> SNAPRRSIHLSNIVEQRVFEDDEIISTPKRGRSKKTVQDNDEDYSPKKSVQKTPTRTRRSSTTTKTATTPSKGITTATATPMTPSQKMKKIRAGELSPSMQQRTDLPAKDSSKSELQLAREQLHVSVVPKSLPCREREFENIYAFLEGKIQDQCGGCMYVSGVPGTGKTATVTGVIRTLQRMAKQNELPAFEYLEINGMRLTEPRQAYVQIYKQLTGKTVSWEQAHALLEKRFTTPAPRRVTTVLLVDELDILCNRRQDVVYNLLDWPTKSAAKLVVVTIANTMDLPERLLMGKVTSRLGLTRLTFQPYSHKQLQEIVTARLGGSETFKGEAVQLVARKVAAVSGDARRALDICRRATEIADTAAVKCVTMLHVQQALAEMIASAKVQAIRNCSRMEQIFLQAIAAEVTRTGVEETTFMGVYQQVETIAAFMGVTFPPPGRALRLCSKLGAERLIISEHSRNDLFQKILLNVSADDIHYALRVEEMVN;> MSASNKGGYKTPRKENLMSIENLTNSEEESEDLNTAMVGNAVESQPKVTSRRSTRRPSPTKKYQAYQKESNGKGQEERIVVNYVEMSDERSSDAEDQEEEESIEESENAARPAAKDLHLIQSEYNVAGTSMFGFNTPKKRDAMALAALNATPCTPKTPKTPRLGVKTPDTKRKKSMDQPKTPAHVRTRVKKQIAKIVADSDEDFSGDESDFRPSDEESSSSSSSSDAGNSSDNDAADDEPKTPSRARRAIVVPVLPKTPSAARLRQSARAKKSNEFVPESDGYFHSHASSKILTSDHTLDRLKNPRLAADRVFSLLSEIKTSAEHEGSINAIMEEYRSYFPKWMCILNEGFNILLYGLGSKHQLLQSFHREVLHKQTVLVVNGFFPSLTIKDMLDSITSDILDAGISPANPHEAVDMIEEEFALIPETHLFLIVHNLDGAMLRNVKAQAILSRLARIPNIHLLASIDHINTPLLWDQGKLCSFNFSWWDCTTMLPYTNETAFENSLLVQNSGELALSSMRSVFSSLTTNSRGIYMLIVKYQLKNKGNATYQGMPFRDLYSSCREAFLVSSDLALRAQLTEFLDHKLVKSKRSVDGSEQLTIPIDGALLQQFLEEQEKK;> MDPTISVSKGCFVYKNGATRAGKKAASKRKRPAAESSSLLGKEVVQQPFYEEYRKAWNQINDHIADLQHRSYARTLEQLVDFVVGQAERDTPDEVLPTAALLTGINQPDHLSQFTALTQRLHAQRAAMVCVLQSRDCATLKAAVETLVFGLVEDNAEVEQMEDEDEDEDGAERDRKRLRRSQCTMKQLKSWYTNNFDSEQKRRQLVVILPDFECFNASVLQDLILILSAHC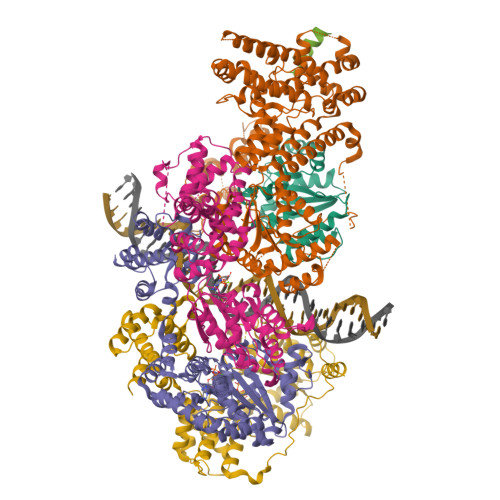GSLPFVLVLGVATAMTAVHGTLPYHVSSKIRLRVFQTQAAPTGLNEVLDKVLLSPKYAFHLSGKTFKFLTHIFLYYDFSIHGFIQGFKYCLMEHFFGGNAFALCTDYSKALGRIKQLTHEDMETIRRLPSFRPYVEQINDCKRIIAVLTDDDYLKKKLPQLLRDCLLHFLLFRCSLEFLTELVGDLPRCPLGKLRRELYVNCLNRAIISTPEYKECLQMLSFLSKDEFVAKVNRALERTEQFLVEEIAPLELGEACTAVLRPKLEAIRLAVDEVVKATMATITTTSPNETRQATDHLTPVASRQELKDQLLQRSKEDKMRHQLNTPTTQFGRALQKTLQLIETQIVQDHLRALQDAPPIHELFVFSDIATVRRNIIGAPRAALHTALNNPHFYMQCKCCELQDQSLLVGTLPDLSVVYKLHLECGRMINLFDWLQAFRSVVSDSDHEEVAQEQIDPQIQARFTRAVAELQFLGYIKMSKRKTDHATRLTW;> SNAMPEADRELVSIRRFLKERLQRDYTTLRGYAKERSNVRLLLQRTAEMGESNSLLLLGPRGSGKTTLINSVLADLLPNKSFGENTLIVHLDGNLHTDDRVALKSITVQMQLENAADGKVFGSFAENLAFLLQCLKAGGKHSKSVIFILEEFDLFCAHHNQTLLYNLFDVSQSAQAPICVLGVTCRLDVIELLEKRVKSRFSHRQVFLFPSLRRFEDYVDLCRDLLSLPTGNSLLLAAEKIYNLQNIQSGALYFSRNHFDPGEYGFSPRLRDAWNKQICKVLATQQARSTLQALHDFDISEAYLKNFLFRLVAHLRPQSPHITAEKMAAVGSQFEGDDKIELLCGLSVLELCLIIAIKHHSQIYDRDSFNFEIIYARFSKFAKVSTTMQAVERSIVLKAFEHLRIAELIMPLTGGAGGGVGKVQKEFEMHKLALTYSQIHHCMQRYQALPTEVAQWAQSSLI;> MEAICSSLEPLFPCREAAIETLGELIGDSSETYPSAIYLFGHSGTGKTALTRAFLKECGKRQNVRTAHLNAIECYTTKIMLEILLDSLAPDQGDALKVDNMLDFVEQLRRQAATRVEDQGFLIAVDNAERLRDMDANVLPVLLRLQELTNLNLCVILLSQLPFEKFYNKTGLSEIVCLHLAQYNKAETQRILGSDFQQVRNQLLEQFAQDKKRLEICQEAVTEDFYNNYLNLFLSVFYKACRDVPELQLTARKCLSTYLEPVLDGTVDATDISRLWRHIAGPLRSALTQIYMRIEKPAEEVEDFTAIEDQSVRKLAQSLELPYYAKFLLIAAFLASHNAAKQDKRLFVKHHGKQRKRMQTVNARAKTTEKMSTTLGPKSFSIDRLLAIFYAILEEKVGLTCNLLSQISTLVHLNLLSFVSGEQNIMEGSARLQCTIGLEFVLQIGKVVGFNVRQYLCDFM;> MTTLIEQLITKMGLREEPNVLEKTTELVRLLELRSTNVPLQINEYGKIVLCADLASCMIGIAFDKEQALKLSGLRKSQYLNNKRMFEKLLDLNKLASVNDICVQLGLNEVARKAEELMTLFKGVAATEDMGTDTSHPQYATMAVFQACRLLKKKVSKSKLMPFSNLRPSQFQLLEQQWERMIAKHHKESKVPSSTDMEGKLKENQNENIKGHEAKKAHKPPPEDYEIWKARMLAKAQAKLKELEASQSHMDSQLLEA2-[1-(4-chlorobenzene-1-carbonyl)-5-methoxy-2-methyl-1H-indol-3-yl]-N-[2-({[5-(dimethylamino)naphthalen-1-yl]sulfonyl}amino)ethyl]acetamide | C33 H33 Cl N4 O5 S | 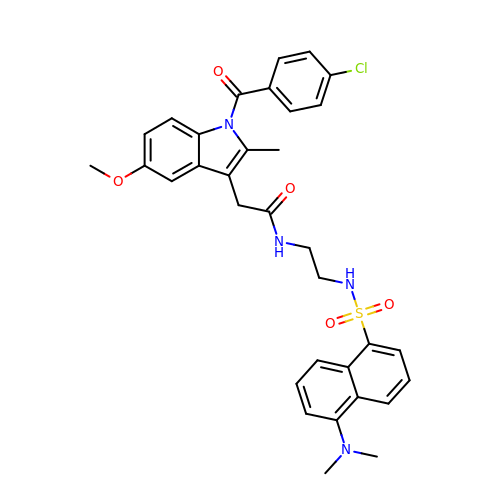GWNNEESLGDFXNP-UHFFFAOYSA-N> APARGTLLTSNFLTSYTRDAISAMLASGSQPASGSQPEQAKCNVRVAEFTYATIGVEGEPATASGVLLIPGGERCSGPYPLLGWGHPTEALRAQEQAKEIRDAKGDDPLVTRLASQGYVVVGSDYLGLGKSNYAYHPYLHSASEASATIDAMRAARSVLQHLKTPLS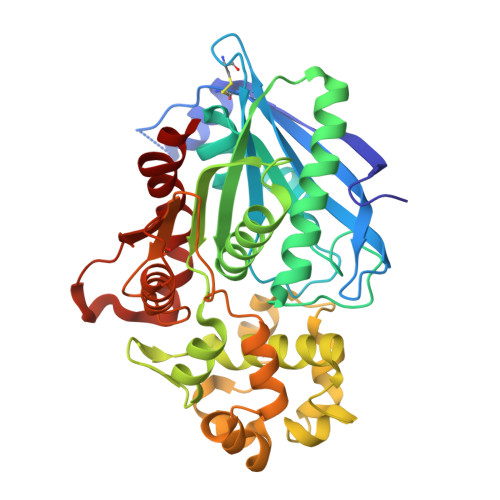GKVMLSGYSQGGHTAMATQREIEAHLSKEFHLVASAPISGPYALEQTFLDSWSGSNAVGEWTFGILLGSYAIVAMQHTYKNIYLEPGQVFQDPWAAKVEPLFPGKQSLTDMFLNDTLPSIDKVKSYFQPGFYSDFPSNPANPFRQDLARNNLLEWAPQTPTLLCGSSNDATVPLKNAQTAIASFQQRGSNQVALVDTGTGNASDNSAFAHMLTKESCIVVVRDQLLDKQR>[3x]ISERDAVKTAISLVGTILGKLGVPLVGPIVSLYSTLIDVLWPGGKSQWEIFMEQVEALINQKIAEYARAKALAELEGLGNNYQLYLTALEEWQENPSSTRVLRDVRNRFEILDSLFTQYMPSFRVTGYEVPLLSVYAQAANLHLLLLKDASIFGEEWGFSTTAINNYYNRQMSLIAQYSDHCVQWYRTGLDRLKGSNAKQWVEYNRFRREMTLSVLDIMTLFPMYDMRTYPMETKAQLTREVYTDPIGAIGAQGSWYDSAPSFNTLESTFIRGKHLFDFITRLSIYTGRSSFSASNYLKKWIGHQISSQPIGGSIQTQTYGTTSGSSVIATQQIGFTGFDVYKTLSTAGVLFAYTSKYYGVSKVVFDAIYPDNKYKTTFTYNPGSEGIGAQEKDSEVELPPETLDQPNYEAY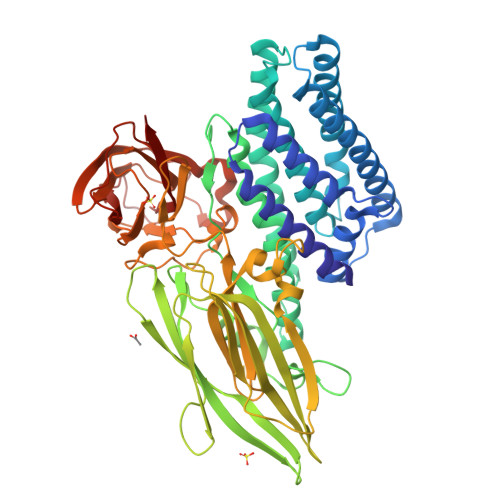SHRLNYVTFIRNPDVPVFSWTHRSADRTNTVYSDKITQIPVVKASDGPKPSANEVGHYLGGDPISFNSSGSTGVIRLNINSPLSQKYRVRIRYCSSVDFDLDVVRGGTTVNNGRFNKSAPNVGWQSLKYENFKFASFSTPFTFNQAQDTLKISVRNFSSIVGGSVVYIDRIELIPVN(5S)-2-amino-5-(2',5'-difluorobiphenyl-3-yl)-3-methyl-5-pyridin-4-yl-3,5-dihydro-4H-imidazol-4-one 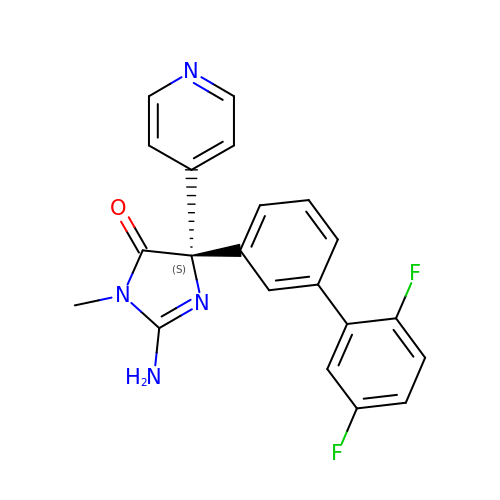| C21 H16 F2 N4 O | RKYFABJLGJZOBA-OAQYLSRUSA-N> GHMRRELAIEFSRVTESAALAGYKWLGRGDKNTADGAAVNAMRIMLNQVNIDGTIVIGEGEIDEAPMLYIGEKVGTGRGDAVDIAVDPIEGTRMTAMGQANALAVLAVGDKGCFLNAPD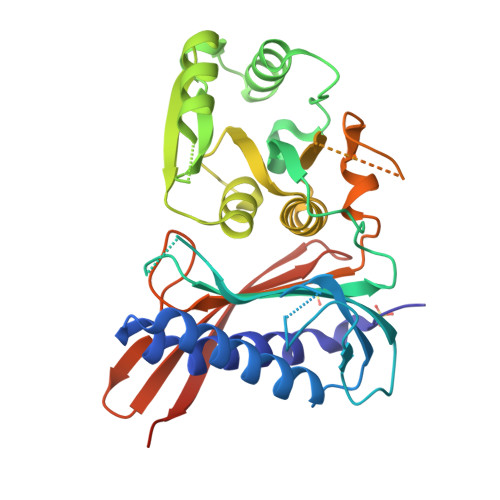MYMEKLIVGPGAKGTIDLNLPLADNLRNVAAALGKPLSELTVTILAKPRHDAVIAEMQQLGVRVFAIPDGDVAASILTCMPDSEVDVLYGIGGAPEGVVSAAVIRALDGDMNGRLLARHDVKGDNEENRRIGEQELARCKAMGIEAGKVLRLGDMARSDNVIFSATGITKGDLLEGISRKGNIATTETLLIRGKSRTIRRIQSIHYLDRKDPEMQVHIL>MNQSSLLAEFGDPITRVENALQALREGRGVLLLDDEDRENEGDIIYAVESLTTAQMALMIRECSGIVCLCLTEAQADRLALPPMVVNNNSANQTAFTVSIEAKHGVTTGVSAQDRVTTIKTAANPQAKPEDLARPGHVFPLRARAGGVLARRGHTEGTVDLMQMAGLQPAGVLCELTN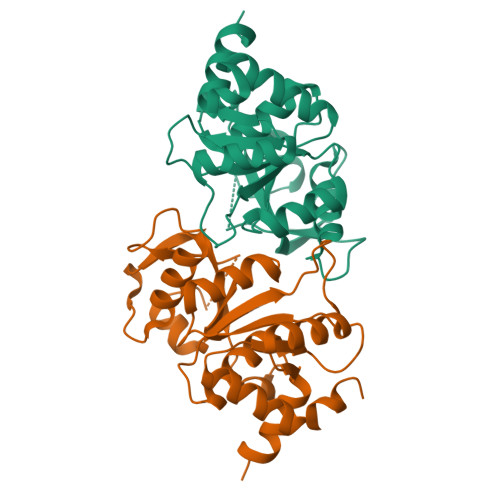PDGSMAKTPEIIEFGKLHNMPVLTIEDMVQYRIQFDLKLA[2x]> MPIFRFTALAMTLGLLSAPYNAMAATSNPAFDPKNLMQSEIYHFAQNNPLADFSSDKNSILTLSDKRSIMGNQSLLWKWKGGSSFTLHKKLIVPTDKEASKAWGRSSTPVFSFWLYNEKPIDGYLTIDFGEKLISTSEAQAGFKVKLDFTGWRAVGVSLNNDLENREMTLNATNTSSDGTQDSIGRSLGAKVDSIRFKAPSNVSQGEIYIDRIMFSVDDARYQWSDYQVKTRLSEPEIQFHNVKPQLPVTPENLAAIDLIRQRLINEFVGGEKETNLALEENISKLKSDFDALNIHTLANGGTQGRHLITDKQIIIYQPENLNSQDKQLFDNYVILGNYTTLMFNISRAYVLEKDPTQKAQLKQMYLLMTKHLLDQGFVKGSALVTTHHWGYSSRWWYISTLLMSDALKEANLQTQVYDSLLWYSREFKSSFDMKVSADSSDLDYFNTLSRQHLALLLLEPDDQKRINLVNTFSHYITGALTQVPPGGKDGLRPDGTAWRHEGNYPGYSFPAFKNASQLIYLLRDTPFSVGESGWNNLKKAMVSAWIYSNPEVGLPLAGRHPFNSPSLKSVAQGYYWLAMSAKSSPDKTLASIYLAISDKTQNESTAIFGETITPASLPQGFYAFNGGAFGIHRWQDKMVTLKAYNTNVWSSEIYNKDNRYGRYQSHGVAQIVSNGSQLSQGYQQEGWDWNRMQGATTIHLPLKDLDSPKPHTLMQRGERGFSGTSSLEGQYGMMAFDLIYPANLERFDPNFTAKKSVLAADNHLIFIGSNINSSDKNKNVETTLFQHAITPTLNTLWINGQKIENMPYQTTLQQGDWLIDSNGNGYLITQAEKVNVSRQHQVSAENKNRQPTEGNFSSAWIDHSTRPKDASYEYMVFLDATPEKMGEMAQKFRENNGLYQVLRKDKDVHIILDKLSNVTGYAFYQPASIEDKWIKKVNKPAIVMTHRQKDTLIVSAVTPDLNMTRQKAATPVTINVTINGKWQSADKNSEVKYQVSGDNTELTFTSYFGIPQEIKLSPLP

Chondroitinase ABC I (cABC-I) is the enzyme which cleaves the β-1,4 glycosidic linkage of chondroitin sulfate (CS) by β-elimination. A 997-amino acid residue monomeric protein, cABC-I, is an endolytic enzyme with broad reactivity to CS isomers as substrates. CS is a sulfated polysaccharide composed of repeating of D-glucuronic acid (GlcA) and N-acetyl galactosamine (GalNAc) with a β1–3 linkage. Recently, cABC-I was used to treat lumbar disc herniation.

The structures of ligand-free cABC-I and cABC-I in complex with disaccharides (ΔDi-4S, ΔDi-6S or ΔDi-0S), the final product of the enzymatic reaction, have been determined at 1.88 Å, 1.80 Å, 1.92 Å and 2.50 Å resolutions, respectively. The overall structures of cABC-I bound to these disaccharides were almost identical to those of the unbound form (Cα r.m.s.d.: cABC-I-ΔDi-4S complex, 0.131 Å; cABC-I-ΔDi-6S complex, 0.161 Å; cABC-I-ΔDi-0S complex, 0.217 Å), indicating that cABC-I was not conformationally changed by interaction with disaccharides. However, the crystal structure of cABC-I in complex with its substrates has never been determined.>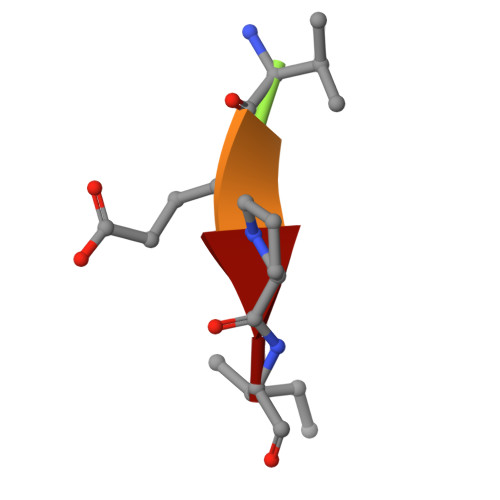 XVEPI>MGGSVIVIDSKAAWDAQLAKGKEEHKPIVVDFTATWCGPCKMIAPLFETLSNDYAGKVIFLKVDVDAVAAVAEAAGITAMPTFHVY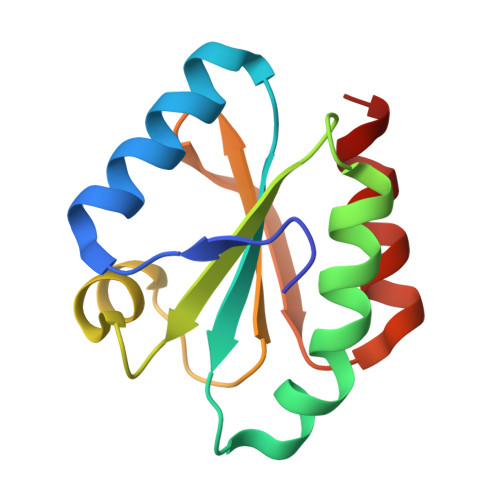KDGVKADDLVGASQDKLKALVAKHAAA[2x]>[2x]MIVLALDVYEGE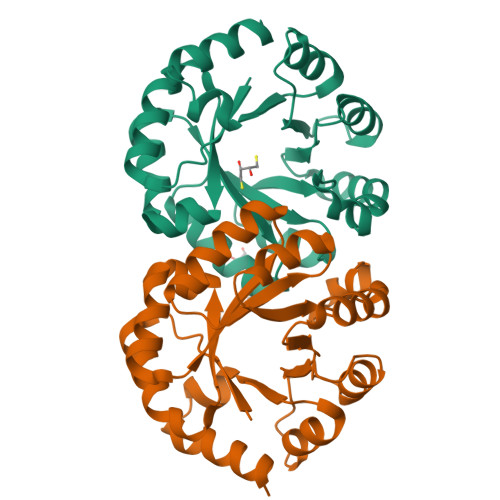RAIKIAKSVKDYISMIKVNWPLILGSGVDIIRRLKEETGVEIIADLKLADIPNTNRLIARKVFGAGADYVIVHTFVGRDSVMAVKELGEIIMVVEMSHPGALEFINPLTDRFIEVANEIEPFGVIAPGTRPERIGYIRDRLKEGIKILAPGIGAQGGKAKDAVKAGADYIIVGRAIYNAPNPREAAKAIYDEIRGV>[2x]MEEECRVLSIQSHVIRGYVGNRAATFPLQVLGFEIDAVNSVQFSNHTGYAHWKGQVLNSDELQELY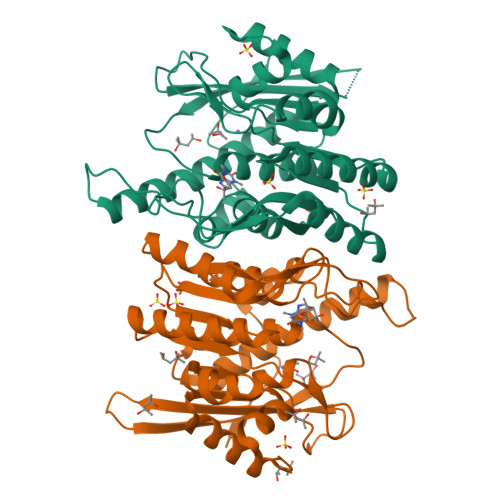EGLRLNNMNKYDYVLTGYTRDKSFLAMVVDIVQELKQQNPRLVYVCDPVLGDKWDGEGSMYVPEDLLPVYKEKVVPLADIITPNQFEAELLSGRKIHSQEEALRVMDMLHSMGPDTVVITSSDLPSPQGSNYLIVLGSQRRRNPAGSVVMERIRMDIRKVDAVFVGTGDLFAAMLLAWTHKHPNNLKVACEKTVSTLHHVLQRTIQCAKAQAGEGVRPSPMQLELRMVQSKRDIEDPEIVVQATVL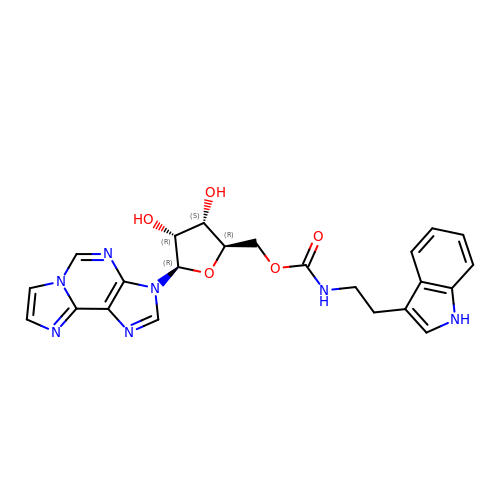[(2~{R},3~{S},4~{R},5~{R})-5-imidazo[2,1-f]purin-3-yl-3,4-bis(oxidanyl)oxolan-2-yl]methyl ~{N}-[2-(1~{H}-indol-3-yl)ethyl]carbamate | C23 H23 N7 O5 | PDQVMZAZVYVBOK-WGQQHEPDSA-N> CLDFNISLAMAKERAHQKRSSKRAPQMDWSK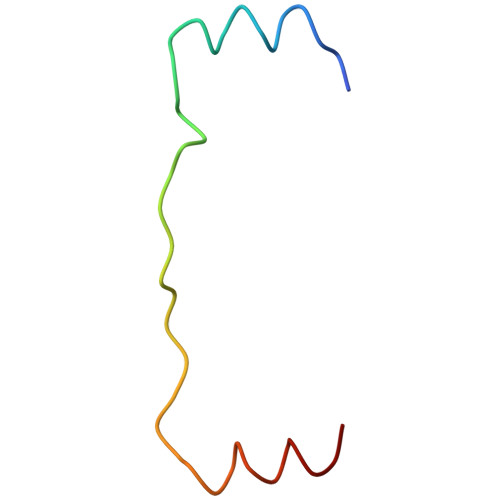KNELFSNL> REFTIDFSTQQSYVSSLNSIRTEISTPLEHISQGTTSVSVINHTPPGSYFAVDIRGLDVYQARFDHLRLIIEQNNLYVAGFVNTATNTFYRFSDFTHISVPGVTTVSMTTDSSYTTLQRVAALERSGMQISRHSLVSSYLALMEFSGNTMTRDASRAVLRFVTVTAEALRFRQIQREFRQALSETAPVYTMTPGDVDLTLNWGRISN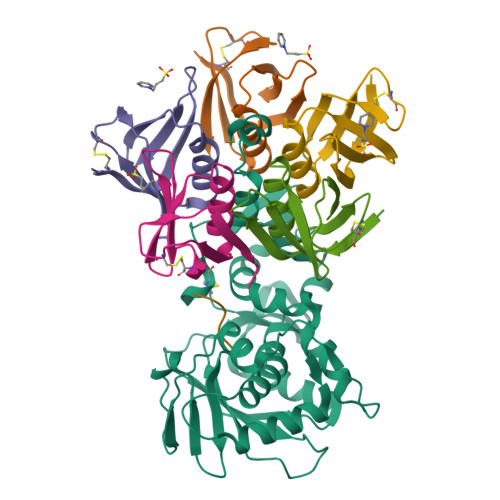VLPEYRGEDGVRVGRISFNNISAILGTVAVILNCHHQGARSVRAVNEESQPECQITGDRPVIKINNTLWESNTAAAFLNRKSQFLYTTGK;>[5x]ADCAKGKIEFSKYNEDDTFTVKVDGKEYWTSRWNLQPLLQSAQLTGMTVTIKSSTCESGSGFAEVQFNND;> MAMMXRRRRAX>MNDNVAWFKQAKYGMMIHWGLYSLLAGEYRGESSSAYAEWIQSKFQIPNAEYGNLATAFNPLYFDAKKIVALAKQCGMQYLVVTTKHHDGFAMYHSKVDAYNVYDATPFHRDIIGELAEACQKAGLKFGLYYSQDLDWHDPNGGGYKSNDVETAGTTWDNSWDFPDEDQKNFDLCFDNKILPQIKEIMSNYGDIATAWFAVPMTLSEAQSQTIYDTVRELQPNCLINSRLGNGKYDFVSLGDNEIPKNKEDMNKTDVDYNEITGFKPSPLGLYETAGTINDSWGFSYHDQNWKTPRTLYRYKQHLNDFGINYLLNVGLDP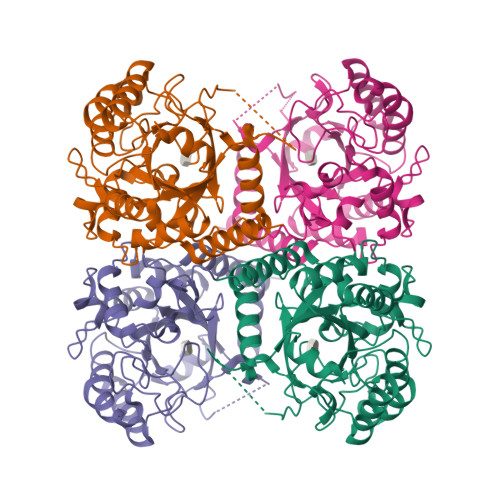LGRVPMMAEENLLAAKALEDEANRL[8x]>[10x]APADNAADAR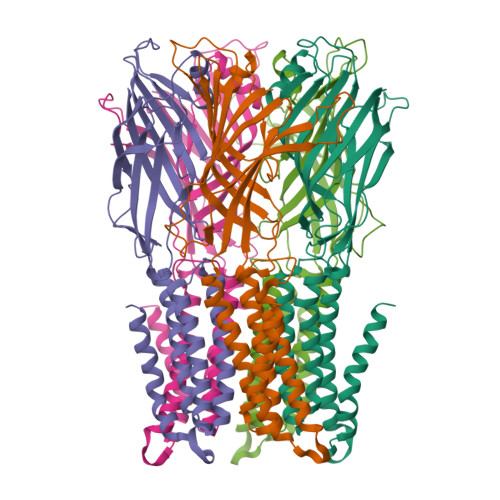PVDVSVSIFINKIYGVNDLEQTYKVDGYIVAQWTGKPRKTPGDKPLIVENTQIERWINNGLWVPALEFINVVGSPDTGNKRLMLFPDGRVIYNARFLGSFSNDMDFRLFPFDRQQFVLELEPFSYNNQQLRFSDIQVYTENIDNEEIDEWWIRGKASTHISDIRYDHLSSVQPNQNEFSRITVRIDAVRNPSYYLWSFILPLGLIIAASWSVFWLESFSERLQTSFTLMLTVVAYAFYTSNILPRLPYTTVIDQMIIAGYGSIFAAILLIIFAHHRQANGVEDDLLIQRCRLAFPLGFLAIGCVLVIRGITL>[4x]GSHMTQQIKLLVLNGPNLNLLGQREPEVYGSKTLDDII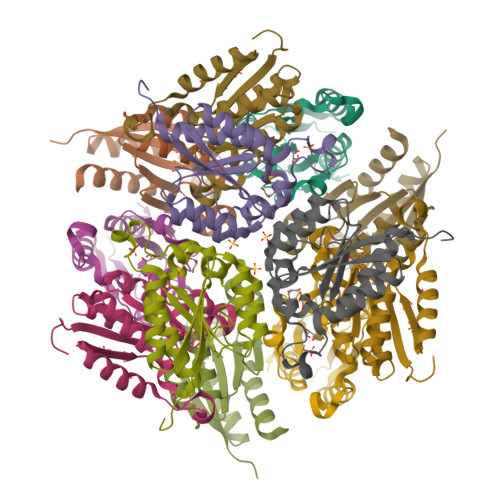KALTDEAALQNVALSHLQSNREYELIEKIHDAFEKIDFIIINPAAFTHTSVALRDALLGVNIPFIEVHLSNVHARESFRHHSYLSDIAQGVICGLGAKGYSFALQSAIGKLRNI>[2x]MSVVPPNRSQTGWPRGVTQFGNKYIQQTKPLTLERTINLYPLTNYTFGTKEPLYEKDSSVAARFQRMREEFDKIGMRRTVEGVLIVHEHRL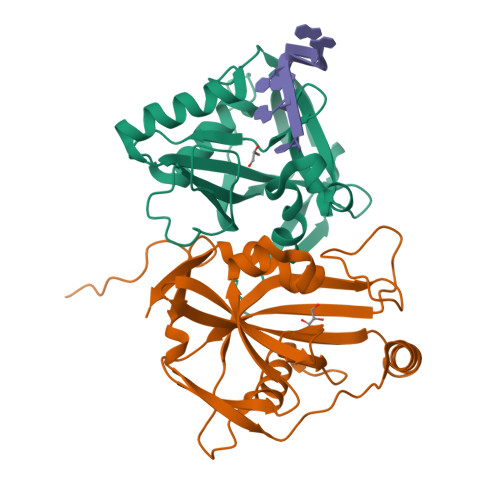PHVLLLQLGTTFFKLPGGELNPGEDEVEGLKRLMTEILGRQDGVLQDWVIDDCIGNWWRPNFEPPQYPYIPAHITKPKEHKKLFLVQLQEKALFAVPKNYKLVAAPLFELYDNAPGYGPIISSLPQLLSRFNFIYN(2S)-2-[6-(methylsulfanyl)naphthalen-2-yl]propanoic acid | C14 H14 O2 S | 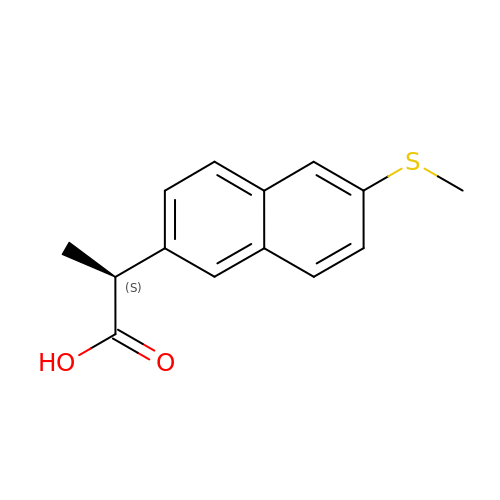DZFJDDMBLJXLJL-VIFPVBQESA-N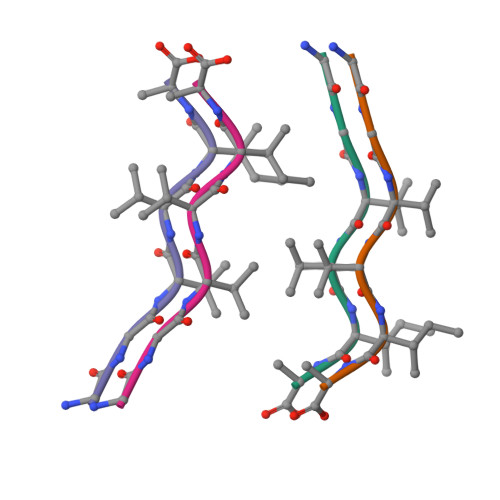> GGVVIA(~{E})-3-[3-(2-methyl-3-phenyl-phenyl)-4-oxidanyl-phenyl]prop-2-enoic 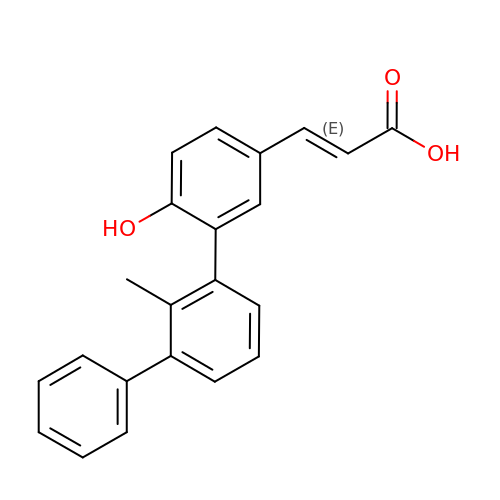acid | C22 H18 O3 | OOQAHTQNBHHYCI-ACCUITESSA-N>[4x]MNTKYNKEFLLYLAGFVDGDGSIIAQIKPNQSYKFKHQLSLTFQVTQKTQRRWFLDKLVDEIGVGYVRDRGSVSDYILSEIKPLHNFLTQLQPFLKLKQKQANLVLKIIEQLPSAKES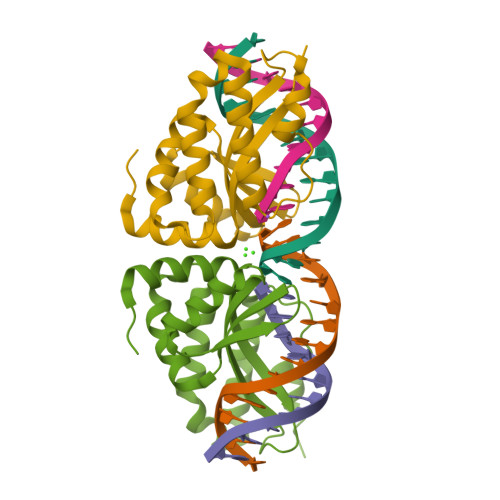PDKFLEVCTWVDQIAALNDSKTRKTTSETVRAVLDSLSEKKKSSP>[2x]GSHMSSLVRRIISTAKAPAAIGPYSQAVLVDRTIYISGQLGMDPASGQLVPGGVVEEAKQALTNIGEILKAAGC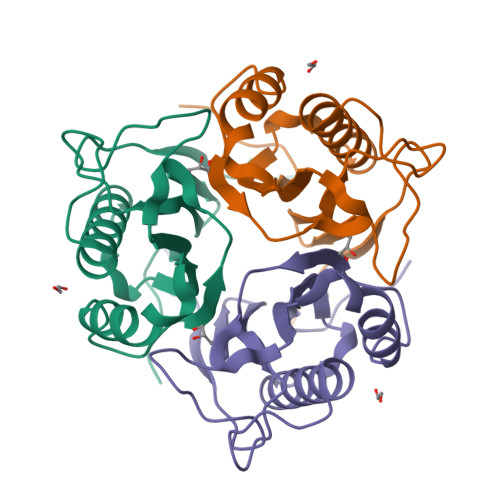DFTNVVKATVLLADINDFSAVNDVYKQYFQSSFPARDAYQVAALPKGGRVEIEAIAVQGPLTTASL> IGTGFPFDPHYVEVLGERMHYVDVGPRDGTPVLFLHGNPTSSYLWRNIIPHVAPSHRCIAPDLIGMGKSDKPDLDYFFDDHVRYLDAFIEALGLEEVVLVIHDWGSALGFHWAKRNPERVKGIACMEFIRPIPTWDEWPEFARETFQAFRTADVGRELIIDQNAFIEGVLPKCVVRPLTEVEMDHYREPFLKPVDREPLWRFPNEIPIAGEPANIVA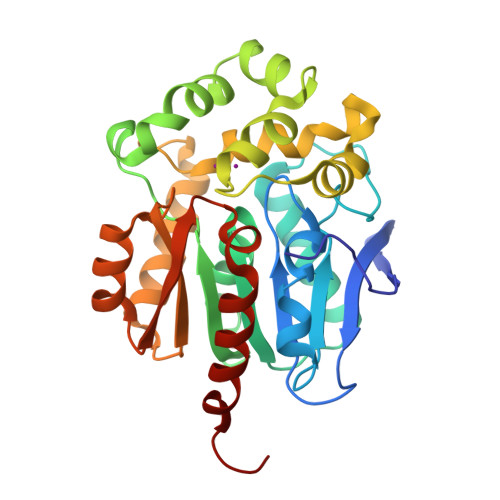LVEAYMNWLHQSPVPKLLFWGTPGVLIPPAEAARLAESLPNCKTVDIGPGLHYLQEDNPDLIGSEIARWLPGLASGLG> A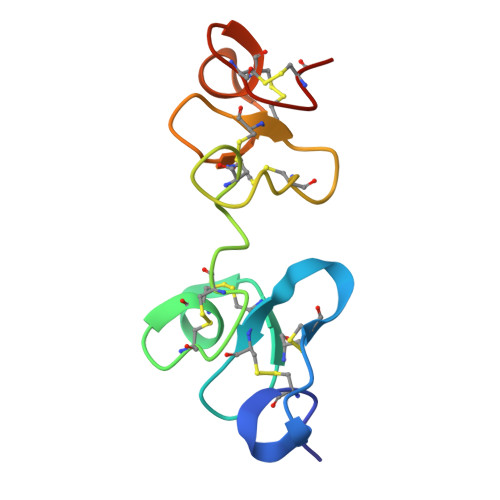PECGERASGKRCPNGKCCSQWGYCGTTDNYCGQGCQSQCDYWRCGRDFGGRLCEEDMCCSKYGWCGYSDDHCEDGCQSQCDLT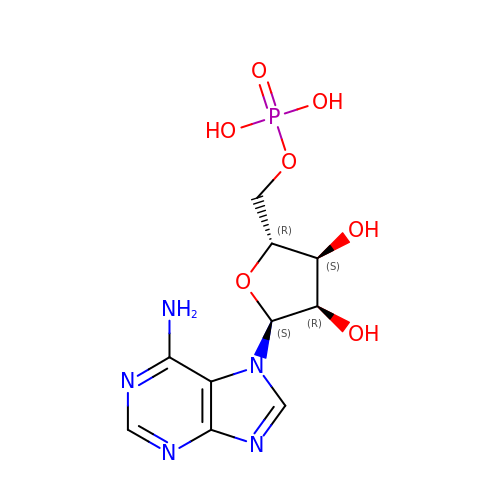ALPHA-ADENOSINE MONOPHOSPHATE | C10 H14 N5 O7 P | NVOIXARBSSLBAS-CRKDRTNXSA-N5'-FLUORO-5'-DEOXYADENOSINE | C10 H12 F N5 O3 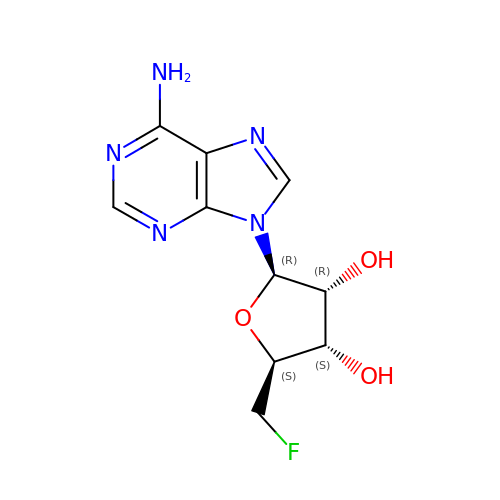| QPVLKMICBYRPSX-KQYNXXCUSA-N>GPGSELPQMVQQLNSPDQQELQSALRKLSQIASGGNEQIQAVIDAGALPALVQLLSSPNEQILQEALWALSNIASGGNEQIQAVIDAGALPALVQLLSSPNEQILQEALWALSNIASGGNEQIQAVIDAGALPALVQLLSSPNEQILQEALWALSNIASGGNEQIQAVIDAGALPA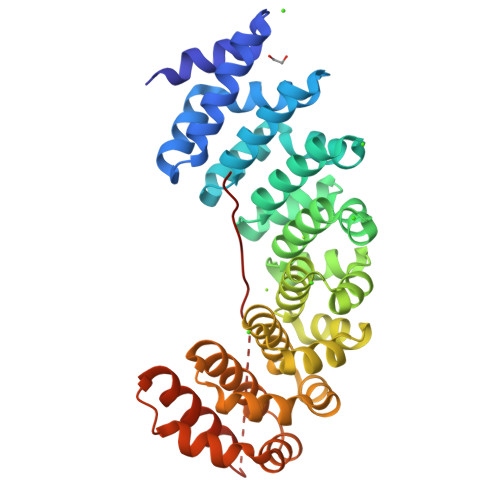LVQLLSSPNEQILQEALWALSNIASGGNEQIQAVIDAGALPALVQLLSSPNEQILQEALWALSNIASGGNEQIQAVIDAGALPALVQLLSSPNEQILQEALWALSNIASGGNEQKQAVKEAGALEKLEQLQSHENEKIQKEAQEALEKLGGGGSGGGGSGKRKRKRKRKRKR[7x];> GPGSELPQMVQQLNSPDQQELQSALRKLSQIASGGNEQIQAVIDAGALPALVQLLSSPNEQILQEALWALSNIASGGNEQIQAVIDAGALPALVQLLSSPNEQILQEALWALSNIASGGNEQIQAVIDAGALPALVQLLSSPNEQILQEALWALSNIASGGNEQIQAVIDAGALPALVQLLSSPNEQILQEALWALSNIASGGNEQIQAVIDAGALPALVQLLSSPNEQILQEALWALSNIASGGNEQIQAVIDAGALPALVQLLSSPNEQILQEALWALSNIASGGNEQKQAVKEAGALEKLEQLQSHENEKIQKEAQEALEKLGGGGSGGGGSGKRKRKRKRKRKRKR N-[(2S)-1-({5-[(diaminomethylidene)amino]pentyl}amino)-1-oxo-3-phenylpropan-2-yl]-4-hydroxy-2-oxo-1,2-dihydroquinoline-6-carboxamide | C25 H30 N6 O4 | 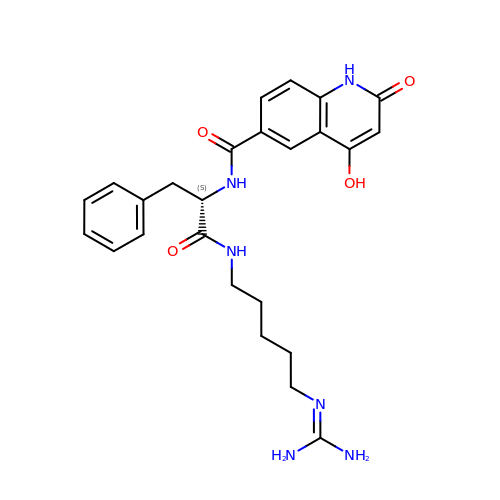YNWDUXLTOPXBFU-FQEVSTJZSA-N(3S)-3-(2,4-dichlorophenyl)-N~1~-hydroxy-N~5~-(3-sulfanylpropyl)pentanediamide | C14 H18 Cl2 N2 O3 S | 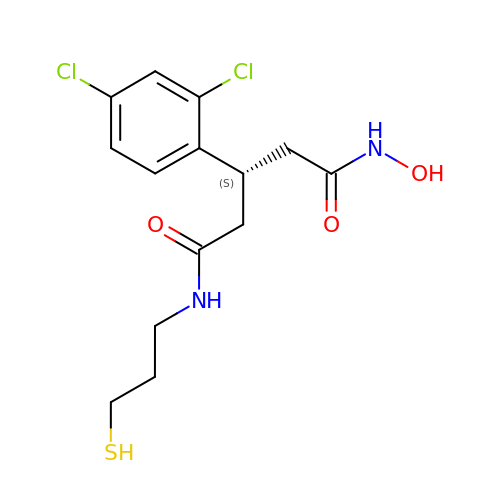IGKGDGVXYQXVLZ-VIFPVBQESA-N>MDNVDFSKDIRDYSGLELAFLGDAIWELEIRKYYLQFGYNIPTLNKYVKAKVNAKYQSLIYKKIINDLDEEFKVIGKRAKNSNIKTFPRSCTVMEYKEA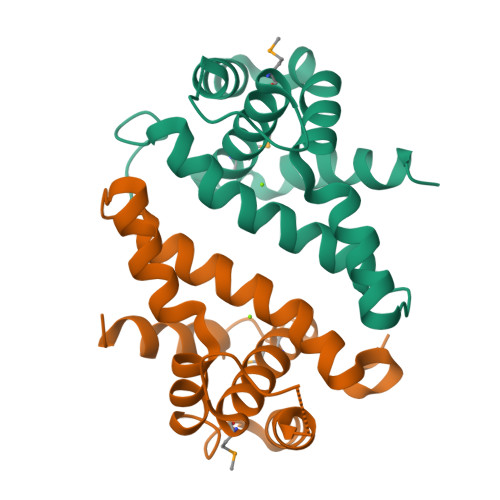TALEAIIGAMYLLKKEEEIKKIINIVIKGELEHHHHHH[6x]>GIDPFTRDGPLVLIGSGLSSEQQKMLSELAVILKAKKYTEFDSTVTHVVVPGDAVQSTLKCMLGILNGCWILKFEWVKACLRRKVCEQEEKYEIPEGPRRSRLNREQLLPKLFDGCYFYLWGTFKHHPKDNLIKLVTAGGGQILSRKPKPDSDVTQT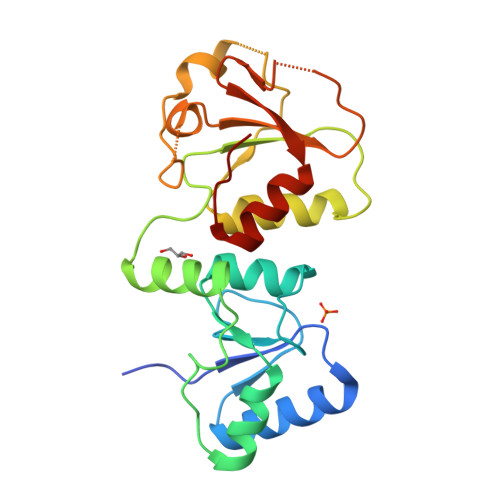INTVAYHARPDSDQRFCTQYIIYEDLCNYHPERVRQGKVWKAPSSWFIDCVMSFELLPLDS[2x]UDP-N-acetyl-muramic acid-4'phosphate 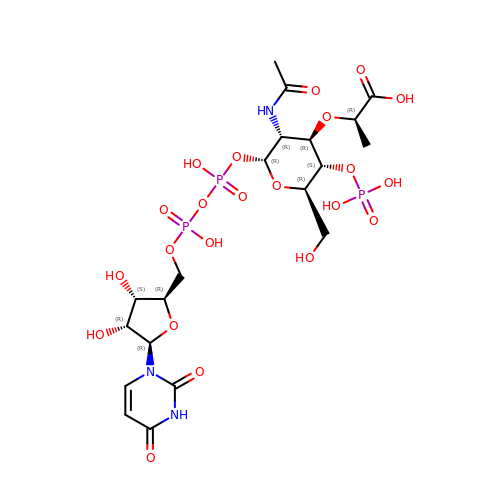| C20 H32 N3 O22 P3 | YABLFTRLTDPKPE-MQTLHLSBSA-N>MGHHHHHHHHHHSSGHIEGRHMMATNLRGVMAALLTPFDQQQALDKASLRRLVQFNIQQGIDGLYVGGSTGEAFVQSLSEREQVLEIVAEEAKGKIKLIAHVGCVSTAESQQLAASAKRYGFDAVSAVTPFYYPFSFEEHCDHYRAIIDSADGLPMVVYNIPALSGVKLTLDQINTLVTLPGVGALKQTSGDLYQMEQIRREHPDLVLYNGYDEIFASGLLAGADGGIGSTYNIMGWRYQGIVKALKEGDIQTAQKLQTECNKVIDLLIK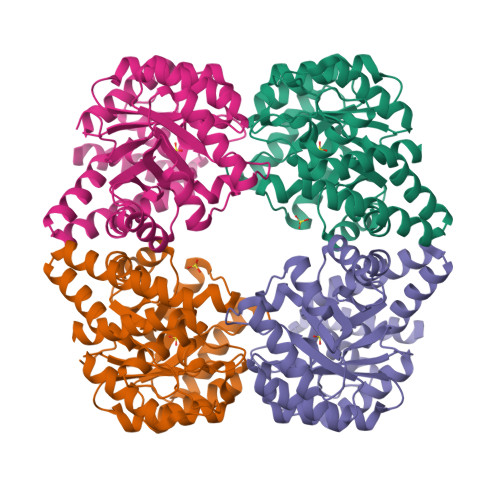TGLFRGLKTVLHYMDVVSVPLCRKPFGPVDEKYLPELKALAQQLMQERG[4x]>MTVEQMMKSGEMIRSVCLGKTKVAEELVNGLRESKFADVKELKCYVNCVMEMMQTMKKGKLNYDASVKQID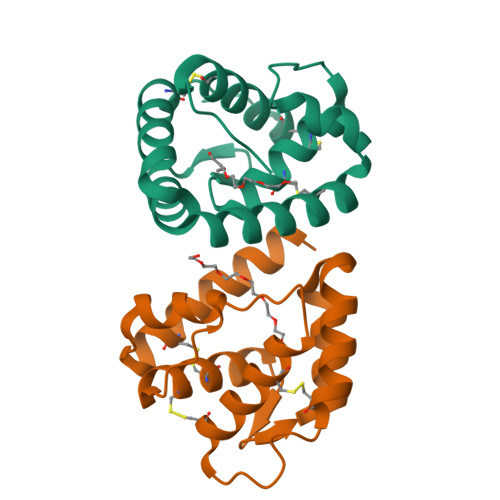TIMPDELAGPMRAALDICRTVADGIKNNCDAAYVLLQCLSKNNPKFIFP[4x]>[3x]PMFIVNT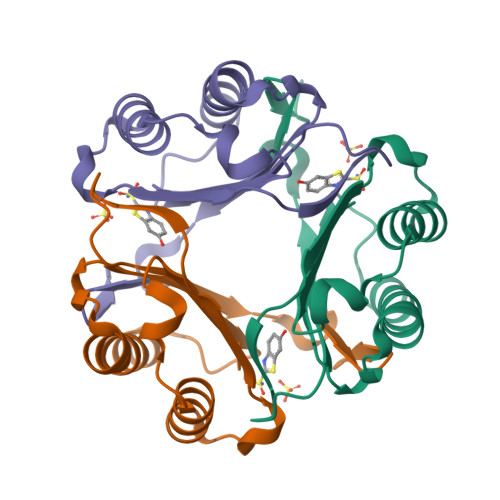NVPRASVPDGFLSELTQQLAQATGKPPQYIAVHVVPDQLMAFGGSSEPCALCSLHSIGKIGGAQNRSYSKLLCGLLAERLRISPDRVYINYYDMNAANVGWNNSTFALEHHHHHH> MERFLLNSTVLLYRLSTVSLDEVSLDERVESSVFLAQYEQARSLPDHVAKSAWSYLVQQIKQRNMKLGPVAILRLIAEKFIKNEKGGPKIDLPMFSEWQTLMSRVSCLPIIACHQVFNPGPASQEYSFRWPLYPYHPTVEDYITRECLHETHQHLNGSTSAEECWLDALKHPEACLRDFEKGWASQEMKQLCAQIDPSLTPRIFKDRLQIACNIREILCRVAQGVELPEWIASMQNPQQLANSTILHNGREYGFATVWPIDDKYSQESEFCWLTGLLEKWRFNAPEGLERLLWIYLLIQNQYLTLLVQRDDFFGFEQFQNYTMTELREETEKSYLSRFKHAHGAGVYSQVRYLEGRFAPKSDPNKMQKLLFSV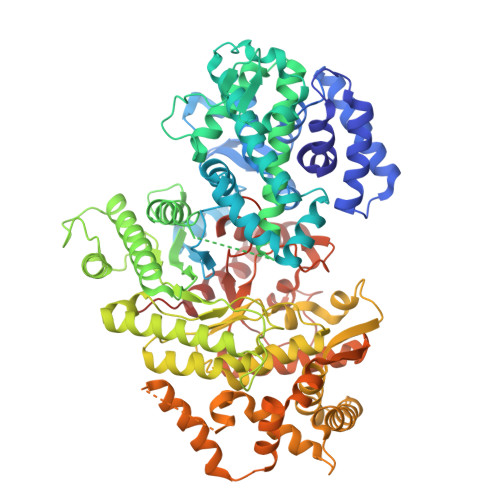LRGYWEYLSAHMSMEWVHEKPLTISQVLDNLELVEPHGKCVELALVPHFIKRKPKNGEAYPHALLFKDLKNQAAILMDMLKSEPRLTGWIRGVDAAANEMHAPPELFCPLFRVLAKSGIAHFTYHVGEDFPHLISGIRSIDDALRFLPLRNGDRLGHCTAIGITPSIWKRSLPLSLSMTKETRLLDLVFIWRELRSHPELLRYASDAAIEAVRLAHKVFSLEEEVSITTLDQVFEMRGLLAESEGLLSELNEPLKPKSLWLEEYERARELVKTTGMKRPLKLYKQWLTSDNVRKQRAEYVEVALEYLPDEAVVALQQAVMAKMADRNIAIECPPTSNTRISQYRNVSEHHIFRWMGLPGEAIEGDVPMSICLGSDDPGIFAADLKSEFYHLFVVLTRKFGLSPADALRKVAEVNENGRIYRFHDVS>GHMNEYFFPKLTAVEALAPYRLRTTWSTGEVLEVDVGDILRKIPDLAPILDPEAFARVHIAEWEGSVEWFDTEFGRDNVYAWAKEQAGEVSHEMFGDWMHRNNLSLTTAAEALGISRRMVSYYRTAHKIIPRTIWLA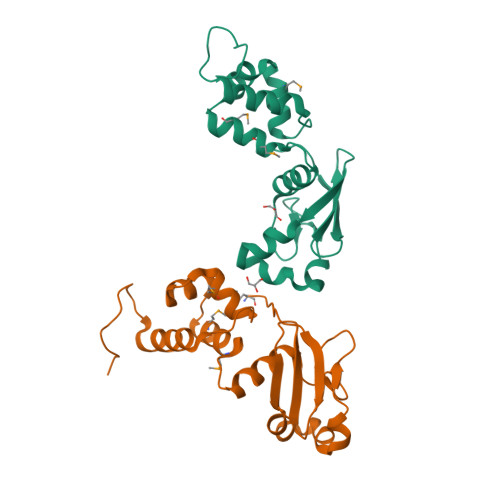CLGWEATRPETKTLPRTLPAAYAKGVSASLSGS[2x]>[2x]GPGADGWLELESDPGLFTLLLKDFGCHDVQVEEVYDLQKPIESPYGFIFLFRWIEERRARRKIVETTAEIFVKDEEAISSIFFAQQVVPNSCATHALLSVLLNCNENNLQLGDTLSRLKTHTKGMSPENKGLAIGNTPELACAHNSHAMPQARRRLERTGAGVSSCRFTGEAFHFVSFVPINGQLFELDGLKPYPMNHGGWEDSEDWTDKFRRVMAERLGIATGEQDIRFNLMAVVPDRRIAITHKLKMLRTNQAIVSGTLQKLLKADEQGESGNGDSQRPDTPTTLLEPSAFTARDLQSLLKNLDTEIAINEQHLADENDRRHMFKVDASRRTHNYDKFICTFLSMLAHQGVLGELVSQHLLPS;>[2x]DGKIDLETPDSILASTNLRALLNKQTFSLLPPLYQYNLIQLLPSVDREASELEQPSSSASGGSPSEAIRLSASCLNNEFFARACLEWRERLSEGEFTPENQLKLKTEAEREKNKLDPWKLKHFEPFWGEKNSRG

The PR-DUB was first characterised in Drosophila melanogaster, where it consists of the deubiquitinase protein Calypso and a binding partner Additional Sex Combs (ASX). The human PR-DUB complex consists of the deubiquitinase Breast Cancer type 1 susceptibility protein (BRCA1)-associated protein-1 (BAP1) and one of three regulatory ASX-Like proteins (ASXL1–3). The PR-DUB complex plays a vital role in regulating H2AK119Ub histone marks, and mutations in human PR-DUB genes lead to a spectrum of malignancies. The overall domain architecture is shared between the human and Drosophila PR-DUB components, with the exception of a large insertion (~380 amino acids) in the ULD domain of BAP1.

With the goal of understanding how PR-DUB activity is coordinated, we have solved the crystal structure of the Drosophila Calypso–ASX complex to a resolution of 3.5 Å. Two copies each of Calypso and ASX are present in the asymmetric unit. In each of the two copies of the Calypso–ASX complex the globular Calypso UCH domain is linked to the C-terminal ULD region by a coiled-coil hairpin. The Deubad domain of ASX packs at the hinge between the coiled-coil and ULD helix of Calypso, restraining the ULD in a pose protruding away from the active site. Whereas Rpn13 consists of seven helices that wrap around the ULD sequence of UCH-L5, only four are defined for ASX. The crystal structure reveals that the NEF-motif sits directly adjacent to ubiquitin in a putative substrate complex. Using size-exclusion chromatography coupled to multi-angle laser light scattering (SEC-MALLS), analytical ultracentrifugation (AUC), small-angle X-ray scattering (SAXS), and chemical crosslinking we demonstrate that Calypso–ASX forms a higher-order complex in solution containing two Calypso and two ASX molecules. Oligomer assembly is mediated by a conserved patch on the surface of the coiled-coil of Calypso, and disruption of this interface impairs recruitment of the PR-DUB to nucleosomes and removal of H2AK119Ub marks. The bidentate Calypso–ASX complex from the crystal structure places two C-terminal tails on the same side of the PR-DUB, with two DUB active sites approximately 60 Å apart.> MGSDKIHHHHHHMKELIRKLTEAFGPSGREEEVRSIILEELEGHIDGHRIDGLGNLIVWKGSGEKKVILDAHIDEIGVVVTNVDDKGFLTIEPVGGVSPYMLL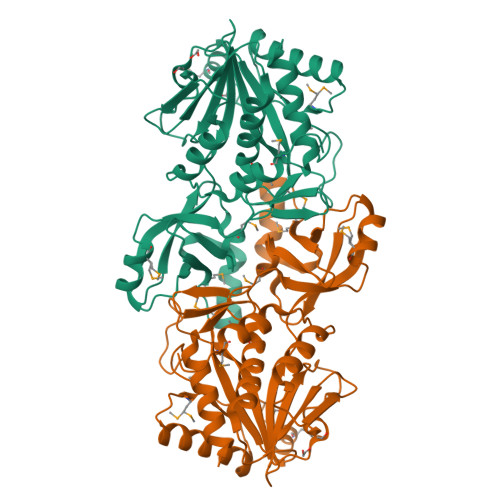GKRIRFENGTIGVVGMEGETTEERQENVRKLSFDKLFIDIGANSREEAQKMCPIGSFGVYDSGFVEVSGKYVSKAMDDRIGCAVIVEVFKRIKPAVTLYGVFSVQEEVGLVGASVAGYGVPADEAIAIDVTDSADTPKAIKRHAMRLSGGPALKVKDRASISSKRILENLIEIAEKFDIKYQMEVLTFGGTNAMGYQRTREGIPSATVSIPTRYVHSPSEMIAPDDVEATVDLLIRYLGA>[4x]MKYMITSKGDEKSDLLRLNMIAGFGEYDMEYDDVEPEIVISIGGDGTFLSAFHQYEERLDEIAFIGIHTGHLGFYADWRPAEADKLVKLLAKGEYQKVSYALLKTTVKYGIGKKEATYLALNESTVKSSGGPFVVDVVINDIHFERFRGDGLCMSTPSGTTAYNKSLGGALMHPSIEAMQLT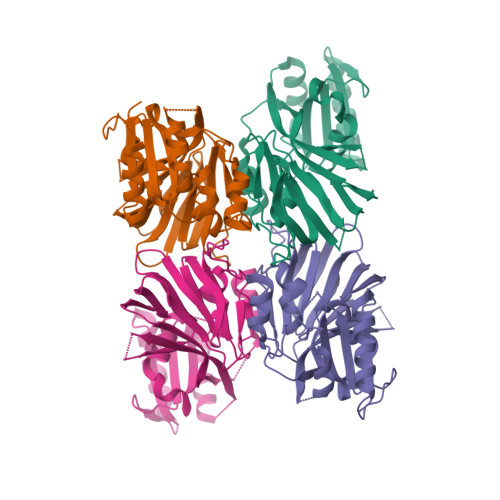EMASINNRVYRTIGSPLVFPKHHVVSLQPVNDKDFQISVDHLSILHRDVQEIRYEVSAKKIHFARFRSFPFWRRVHDSFIEDLEHHHHHH4-HYDROPEROXY-2-METHOXY-PHENOL | 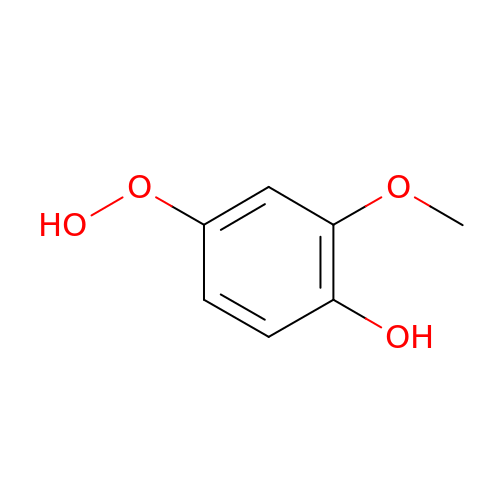C7 H8 O4 | DNBCLSZROQUYQN-UHFFFAOYSA-N>[2x]MKTLSPAVITLLWRQDAAEFYFSRLSHLPWAMLLHSGYADHPYSRFDIVVAEPICTLTTFGKETVVSESEKRTTTTDDPLQVLQQVLDRADIRPTHNEDLPFQGGALGLFGYDLGRRFESLPEIAEQDIV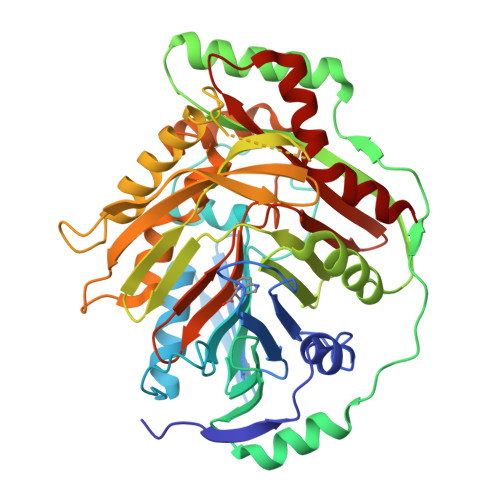LPDMAVGIYDWALIVDHQRHTVSLLSHNDVNARRAWLESQQFSPQEDFTLTSDWQSNMTREQYGEKFRQVQEYLHSGDCYQVNLAQRFHATYSGDEWQAFLQLNQANRAPFSAFLRLEQGAILSLSPERFILCDNSEIQTRPIKGTLPRLPDPQEDSKQAVKLANSAKDRAENLMIVDLMRNDIGRVAVAGSVKVPELFVVEPFPAVHHLVSTITAQLPEQLHASDLLRAAFPGGSITGAPKVRAMEIIDELEPQRRNAWCGSIGYLSFCGNMDTSITIRTLTAINGQIFCSAGGGIVADSQEEAEYQETFDKVNRILKQLEK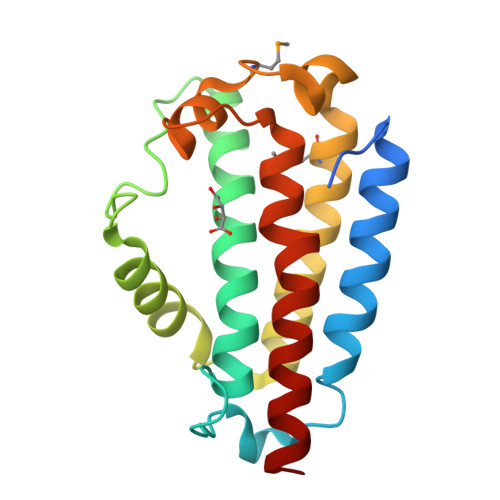>[2x]MRGSHHHHHHGSRVYENKEELKSEINKTFEKYIAEFDNIPESLKDKRIDEVDRTPAENLAYQVGWTTLVLKWEEDERNGLQVKTPSDEFKWNQLGELYQWFTDTYAYLSLQELKSKLNENINSIYVMIDSLSDEELFKPHMRKWADDATKTAVWEVYKFIHVNTVAPFKTFRNKIRKWKKIVL> MCSLDLFPPPLDGSQLPLYEFNNEIVAGKGFDNPPPTFQSELVNIPEPTIPVDALKAPGRMELSSKTAFIHQKESIWKRCLNAWHNVGLAGFLEEMSNSKEEVPPWLCHVTRCSLAVCRSVSSLHGSLFPHLTISPQMKSEDLTAEFSQALGWADCPLRAFAWHPHTYKFALALLDDSIRIYTAGSPTIPTLKHRLQKDVASLAWKPMCASVLAVACQSCVLVWHVDPTSLSTRPSSGCAQVLSHPGHSPVTSVCWSPKGGVLLSASPVDTAMLVWDVPTESCIPLQRVGGGGVTFLSWSPDGSKVLAATPSSVFRVWETQKWTCERWPTLQGRCQTGCWSPDGSRLLFAVKGESVIYSLCFSVSEGEAQAGVGGSQSATVVADVSEVVFTTH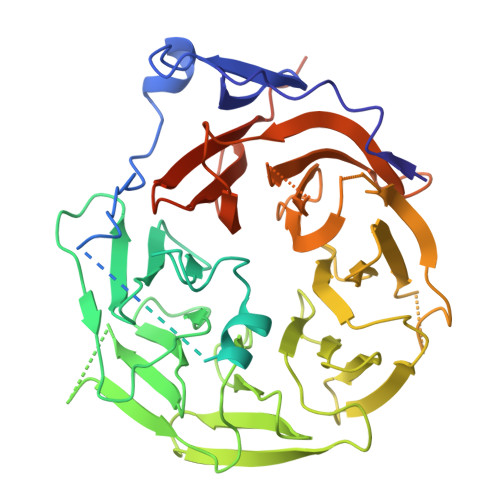TGEIRVGGEIQSMCWDPSGERLAVLLKGNPEFEESQPVIAVFRTRNSPIFELLPCGFIHGRKGETPQLFQFHPGFNKGALLSQLWSSGRVNHFPFYFVNAQCPRFSPESIAVVPGNTISTANPRTLFTER>[5x]TPDCVTGKVEYTKYNDDDTFTVKVGDKELFTNRWNLQS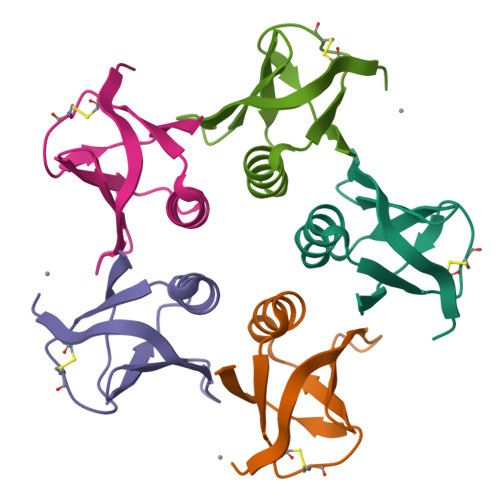LLLSAQITGMTVTIKTNACHNGGGFSEVIFR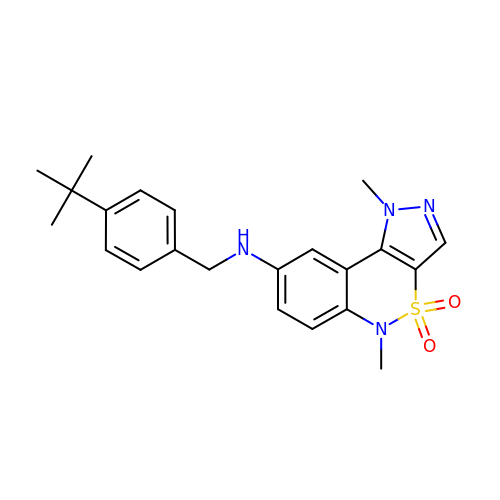N-(4-tert-butylbenzyl)-1,5-dimethyl-1,5-dihydropyrazolo[4,3-c][2,1]benzothiazin-8-amine 4,4-dioxide | C22 H26 N4 O2 S | AVFJKWOKOZKXRX-UHFFFAOYSA-N> NINVDVKQNENDIQVNIAGEIDVYSAPVLREKLVPLAEQGADLRICLKDVSYMDSTGLGVFVGTFKMVKKQGGSLKLEN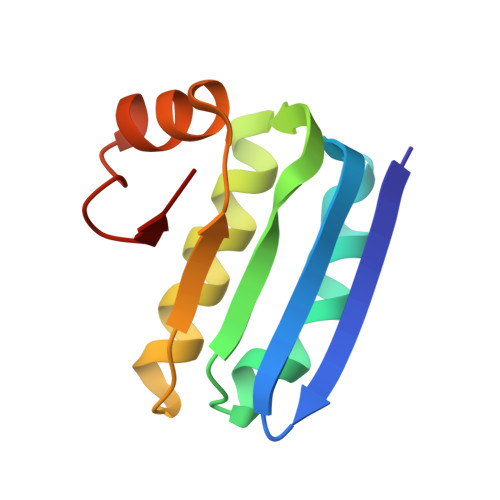LSERLIRLFDITGLKDIIDISAKS> MGCASRDDWRCARSMHEFSAKDIDGHMVCLDKYRGFVCIVTNVASQCGKTDVNYTQLVDLHARYAECGLRILAFPCNQFGRQEPGSNQEIKEFAAGYNVKFDMYSKICVNGDDAHPLWKWMKVQPKGRGMLGNAIKWNFTKFLIDKNGCVVKRYGPMEEPQVIEKDLPCYL

The mammalian glutathione peroxidase (GPx) family is a key component of the cellular antioxidative defence system. Within this family, GPx4 has unique features as it accepts a large class of hydroperoxy lipid substrates and has a plethora of biological functions, including sperm maturation, regulation of apoptosis and cerebral embryogenesis. The mammalian glutathione peroxidase (GPx) family is a key component of the cellular antioxidative defence system. Its eight members (GPx1–GPx8) catalyse the reduction of reactive oxidative species (ROS) such as hydrogen peroxide (H2O2) or other alkyl hydroperoxides at the expense of reduced glutathione and/or other reductants. Among the three different isoforms present in nature, the 170-residue, 19.5 kDa monomeric cytosolic isoform is essential.

In this paper, the structure of the cytoplasmic isoform of mouse phospholipid hydroperoxide glutathione peroxidase (O70325-2 GPx4) with selenocysteine 46 mutated to cysteine is reported solved at 1.8 Å resolution using X-ray crystallography. We successfully cloned, expressed and purified a fragment from Met1 to Leu170 of the cytoplasmic isoform of mouse GPx4 with selenocysteine 46 mutated to cysteine. GPx4 crystallized spontaneously in a 1.5 ml reaction tube at 2 mg ml−1 concentration at room temperature after acquiring the NMR spectrum. The first six N-terminal residues, Met1, Gly (added for the purposes of cloning) as well as Cys2–Arg5, are not visible owing to disorder. Overall, the mouse GPx4 has the same fold as its human homologue. With a root-mean-square deviation (r.m.s.d.) of 0.21 Å for 165 superimposed Cα atoms, the structures can be considered to be isomorphous. The active site of the GPx4 enzyme consists of the catalytic tetrad Sec46, Gln81, Trp136 and Asn137. In this study selenocysteine 46 was mutated to cysteine. The active-site cavity is surrounded by a number of positively charged amino-acid residues (Lys48, Arg80 and Lys135). All of the cysteine residues are in the reduced form.>TVNWEDRPSTPTILGYEVMEERAKFTVYKILVKKTPEESWVVFRRYTDFSRLNDKLKEMFPGFRLALPPKRWFKDNYNADFLEDRQLGLQAFLQNLVAHKDIANCLAVREFLCLDDPPGPFDSLEESRAFCETLEETNYRLQKELLEKQKEME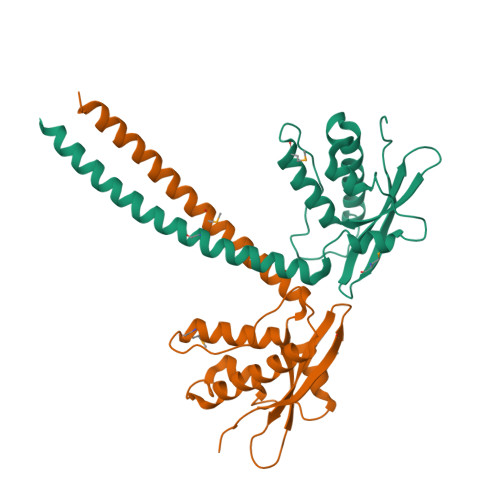SLKKLLSEKQLHIDTLENRIRTLSLE[8x]>[4x]MKGPYKHFMQKEIFEQPDSAFNTMRGRIDFENCVVTLGGLKSWLSTIRRCRRIIMIACGTSYHSCLATRSIFEELTEIPVSVELASDFLDRRSPVFRDDTCVFVSQSGETADSILALQYCLERGALTVGIVNSVGSSMSRQTHCGVHINAGPEIGVASTKAYTSQYIALVMFALSLSNDSISRKGRHEEIIKGLQKIPEQIK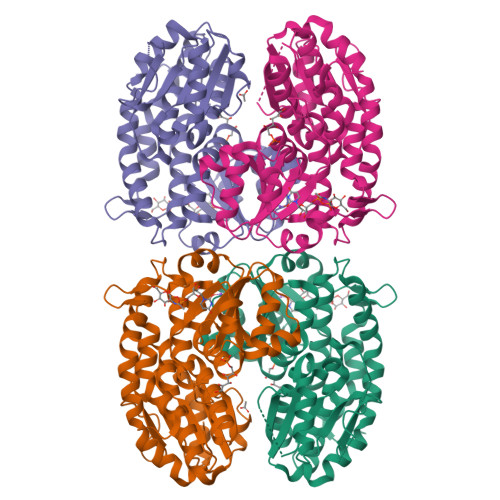QVLKLENKIKDLCNSSLNDQKSLLLLGRGYQFATALEGALKIKEISYMHSEGVLAGELKHGILALVDEDLPIIAFATRDSLFPKVMSAIEQVTARDGRPIVICNEGDAIISNDKVHTTLEVPETVDCLQGLLNVIPLQLISYWLAVNRGIDVDFPRNLAKSVTVE>MTSRGDSREKILHTASRLSQLQGYHATGLNQIVKESGAPKGSLYHFFPNGKEELAIEAVTYTGKIVEHLIQQSMDESS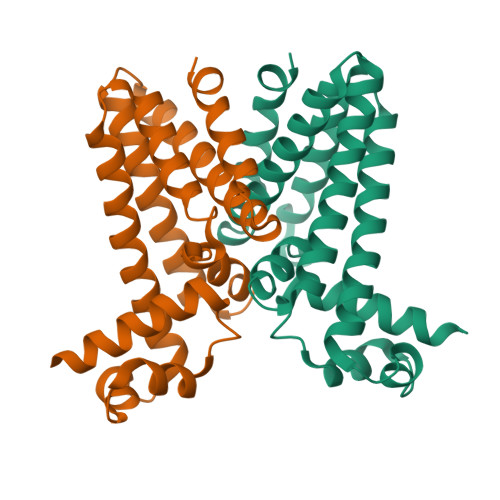DPVEAIQLFIKKTASQFDNTESIKGIPVGLLASETALISEPLRTVCMKVFKSWEAVFARKLMENGFAEEEANQLGTLINSMIEGGIMLSLTNKDKTPLLLIAEQIPVLVRKKG[2x]Macrophage infectivity potentiator (MIP) proteins are key microbial virulence factors that facilitate host cell infection, intracellular pathogen replication, and dissemination. They are found in a variety of pathogens of both bacterial and eukaryotic origin, including Burkholderia pseudomallei, the causative agent of melioidosis, Legionella pneumophila, leading to Legionnaires’ disease, and the protozoan parasites Trypanosoma cruzi and Leishmania subspecies. All MIP proteins share a peptidyl-prolyl-cis–trans-isomerase (PPIase) domain resembling the FK506 binding protein domains of human FKBPs. All MIP and FKBP proteins share a general domain topology in their core PPIase domain with an amphipathic five-stranded β-sheet wrapping around a short α-helix, thereby forming a hydrophobic active site32. Inhibition of secreted MIP proteins diminishes macrophage invasion and leads to the reduction of overall pathogen load and virulence, as shown for L. pneumophila and B. pseudomallei, respectively.

Here, we determined the crystal structures of B. pseudomallei MIP (BpMIP), which contains only the core PPIase domain and T. cruzi MIP (TcMIP), which features the PPIase domain and a free-standing α-helix (“stalk”), in complex with fluorinated pipecolic acid inhibitors. In all cases, we found that the inhibitor molecules bound within the expected FKBP-like domain cleft that forms the MIP active site. For LpMIP100–213, the affinity for the tracer was significantly lower than that for all other constructs, thus requiring a 5-fold increase in the protein concentration. Both NJS224 and NJS227 were able to displace the tracer and yielded displacement KD values in the low to medium nM range for BpMIP and TcMIP and in the low μM range for full-length LpMIP and LpMIP77–213. NJS224 carries a fluorinated thioaryl group (henceforth denoted X1) and an isopropyl group (X2A) and gives rise to a single resonance at −113.19 ppm. In agreement with very similar KD values for either ligand, the distinguishing moieties, i.e., the iso-propyl group in NJS224 and the para-fluorobenzyl moiety in NJS227, do not make substantial protein contacts and furthermore face in opposite directions. A highly similar interaction mode for both inhibitors is also apparent from their nearly identical CSP pattern when bound to 15N-labeled TcMIP. The fluorobenzyl group attached to the sulfoxyl group, i.e., the group present in either inhibitor, is nestled into a hydrophobic pocket formed by F43 in β-strand 3a and V97/I98 in the loop between β4 and β5 in BpMIP and the corresponding residues F73 and M125/I126 in TcMIP. In the crystal structures, the inhibitor’s piperidine ring rests within a hydrophobic cage formed by conserved aromatic residues (Y33/Y63, F53/F85, and W66/W94 in BpMIP and TcMIP, respectively). In BpMIP and TcMIP, hydrophobic residues in this region (V62/I63 in BpMIP and V90/I91 in TcMIP) interact with the inhibitor pyridine group.

> ASHEERMNNYRKRVGRLFMEQKAAQPDAVKLPSGLVFQRIARGSGKRAPAIDDKCEVHYTGRLRDGTVFDSSRERGKPTTFRPNEVIKGWTEALQLMREGDRWRLFIPYDLAYGVTGGGGMIPPYSPLEFDVELISIKDGGKGRTAEEVDEILRKAEEDRED The Vtc4p β-tunnel domain is not unique to eukaryotic polyP polymerases but is a structural hallmark of triphosphate tunnel metalloenzymes (TTMs), whose characteristic features are the presence of a topologically closed hydrophilic β-barrel, the preference for triphosphate-containing substrates, and for a divalent metal co-factor (PFAM families CYTH and VTC). Members of the ancient triphosphate tunnel metalloenzyme family can be found in all kingdoms of life. Our comparative analysis defines that most of these enzymes share a common catalytic mechanism in their tunnel centers, yet they have evolved different substrate recognition modes on their tunnel entries. The observed substrate plasticity apparently allows TTM proteins to act on a wide array of enzyme substrates and to perform very different reactions, many of which likely remain to be discovered.

Instead, AtTTM3 has specific, Mg2+ ion-dependent, short-chain polyphosphatase activity as previously reported. As AtTTM3 efficiently hydrolyzes PPPi in the presence of Mg2+ ions only at neutral or basic pH, we used two crystal forms grown at pH 5.0 (form A) and pH 7.5 (form B) to crystallize substrate-metal complexes under non-hydrolyzable and hydrolyzable conditions, respectively. In both crystal forms, we determined structures of AtTTM3 in the presence of PPPi and either MgCl2 or MnCl2. At pH 5.0 (form A) we find a triphosphate moiety bound in the AtTTM3 active site. Here, PPPi coordinates a Mg2+/Mn2+ ion that acts as a bridge between the substrate and the invariant Glu-169AtTTM3. A short soak at pH 7.0 (form B) shows the same arrangement of PPPi and Mn2+ in the active site. In all our structures the catalytic Mg2+ ions can be substituted by Mn2+ ions, for which we calculated phased anomalous difference electron density maps from data collected near the Mn-K edge to confirm their modeled positions. The basic residues in the tunnel center appear to be mainly involved in substrate coordination; however, the invariant Arg-56ygiF (Arg-52AtTTM3) possibly activates the substrate for the nucleophilic attack by forming a hydrogen bond with the oxygen atom connecting the β- and γ-phosphate of the substrate.

> GAMEVEVKLRLLTAAAHLRLTTLLTPYHLKTLHQRNTFFDTPKNDLSLRRAVLRLRFLQNAAVSAASPSPPRCIVSLKAKPTLANGISRVEEDEEEIEYWIGKECVESPAKLSDIGSRVLKRVKEEYGFNDFLGFVCLGGFENVRNVYEWRGVKLEVDETKYDFGNCYEIECETEEPERVKTMIEEFLTEEKIEFSNSDMTKFAVFRSGKLP INOSINE | C10 H12 N4 O5 | 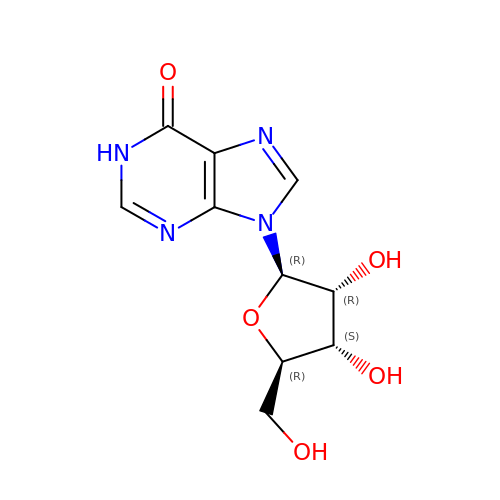UGQMRVRMYYASKQ-KQYNXXCUSA-N N-cyclopropyl-2-methyl-4-(7-{[2-(morpholin-4-yl)ethyl]amino}-5-phenoxypyrazolo[1,5-a]pyrimidin-3-yl)benzamide 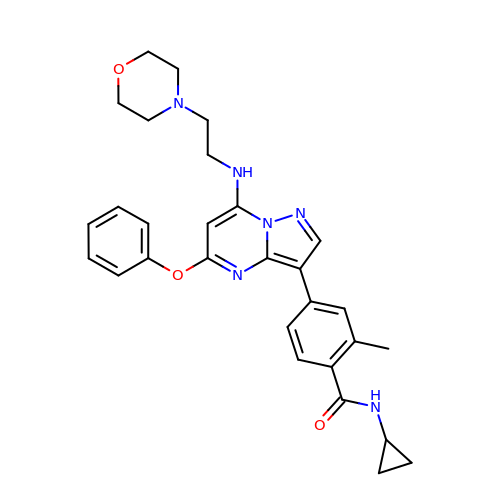| C29 H32 N6 O3 | AKGWVDBXMHMMSD-UHFFFAOYSA-N>[2x]NLYFQGAGAGAGAGAMS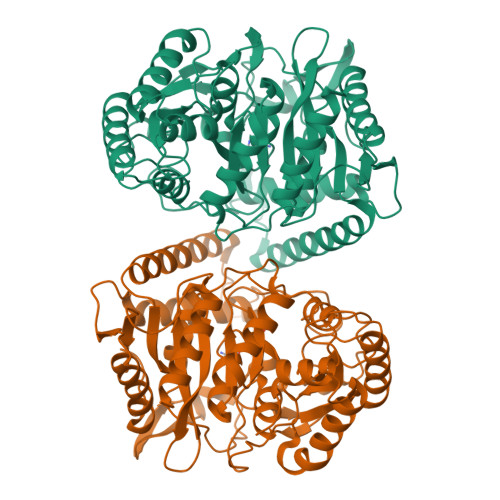ELSAIETAAAIAGGSMTALEACDAAIARIEQRDGPINAVVVRDFDRARDAAKAADAEIAAAVRKPLLGVPMTIKESFDIAGLPTSWGFAEHADHIATADSLVVSRLKAAGAVFLGKSNIPVGLADWQSVNPNYGRTNNPHDHSRSAGGSSGGAAAALAAGMVPLEYGSDIGGSIRVPAHFCGVWGLKTTFDAVSLEGHYFPRTDSAKADLSVVGPMARTPADLALALDITSKVPLPQSRIANLSGLRILLLTAHPETVADSATISAVERAAAACEASGATVATSSPDLPDLSALVADYTRMLLVVLARGLAPEGTEPVSLNAWYAMLDDQARMMRAFDRLFESFDAIFCPVLGTTAFAHSDEPDWAKRSLSIDGGIAPFAAQLGWISMATYGGMPALSMPLGADGNGLPINLQIITRNWSDHDAIRIGALVAEALDR The retroviral structural protein Gag forms the immature protein shell of nascent virus particles4. All retroviral Gag proteins contain three canonical domains: matrix (MA), capsid (CA), consisting of independently folded N-terminal (CA-NTD) and C-terminal (CA-CTD) domains, and nucleocapsid (NC). During immature virus particle formation, these domains function in membrane binding, viral lattice self-assembly and viral genomic RNA (vgRNA) packaging, respectively. Our results show that HTLV-1 uses a distinct CA-NTD arrangement to form the immature Gag lattice and that, in contrast to other retroviral structures, the CA-NTD is the key determinant of immature HTLV-1 assembly.

To analyze the structure of immature HTLV-1 lattice interfaces in more detail, we engineered an HTLV-1 Gag truncation construct for bacterial expression, purification, in vitro assembly and analysis by cryo-ET. The MA126CANC tubes exhibited varying helical parameters. Tubes were sorted into nine groups and each group was processed separately by subtomogram averaging. The two groups with the largest number of tubes had similar geometry and, thus, they were pooled and processed together. The resulting final reconstruction of the CA-NTD layer had an overall estimated resolution of 3.4 Å. The helical pitch and densities for large side chains were clearly visible at this resolution, which enabled us to build a refined model of the immature CA-NTD lattice interactions. The in vitro assembled tubes had the same arrangement of the CA-NTD layer as the full-length HTLV-1 Gag VLPs (Cα root-mean-square deviation (r.m.s.d.) = 1.2 Å), underscoring the biological relevance of our in vitro system. Specifically, CA-NTD residues M17 and Y61 have been identified as essential for immature HTLV-1 Gag lattice assembly and particle formation. In our model, these residues are located in helices 1 and 3, respectively, which form the hexamerization interface together with helix 2. To further characterize this interface, we substituted residue L43, which interacts with M17 and Y61 in our model.

>[3x]PVMHPHGAPPNHRPWQMKDLQAIKQEVSQAAPGSPQFMQTIRLAVQQFDPTAKDLQDLLQYLCSSLVASLHHQQLDSLISEAETRGITGYNPLAGPLRVQANNPQQQGLRREYQQLWLAAFAALP> SLLRFSAVSRHHRGASIDPMTFSEATTPDALTPDAHTPRLLTCDVLYTGMGGAQSPGGVVVVGETVAAAGHPDELRRQYPHAAEERAGAVIAPPPVNAHTHLDMSAYEFQALPYFQWIPEVVIRGRHLRGVAAAQAGADTLTRLGAGGVGDIVWAPEVMDALLAREDLSGTLYFEVLNPFPDKADEVFAAARTHLERWRRLERPGLRLGLSPHTPFTVSHRLMRLLSDYAAGEGLPLQIHVAEHPTELE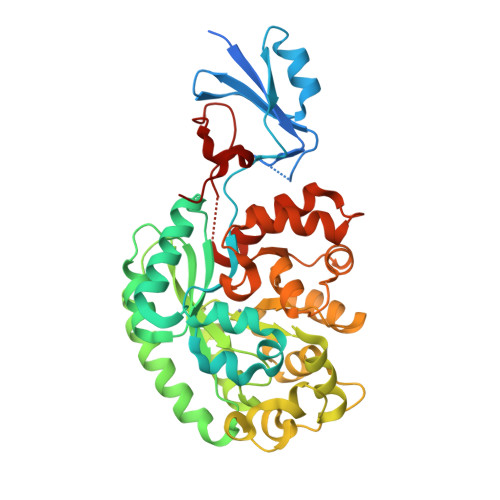MFRTGGGPLWDNRMPALYPHTLAEVIGREPGPDLTPVRYLDELGVLAARPTLVHMVNVTPDDIARVARAGCAVVTCPRSNHHLECGTFDWPAFAAAGVEVALGTDSVASGETLNVREEVTFARQLYPGLDPRVLVRAAVKGGQRVVGGRTPFLRRGETWQEGFRWELSRDL>[2x]MGHHHHHHMVK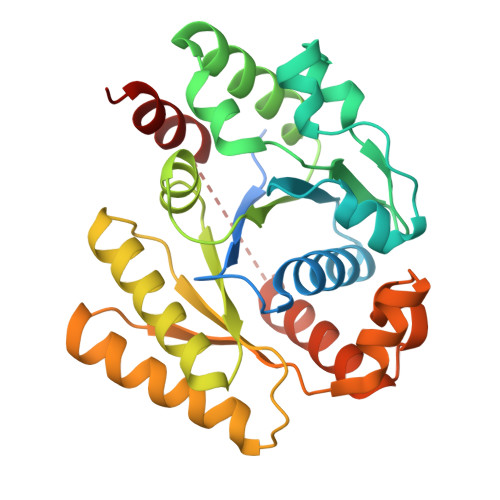DQAEQLRLKLSRLRQQPSPRTIAVTSGKGGVGKSNVSLNFSLSLSKLGFRVLLLDMDIGMGNIDILLGESSSLALADWFSARLPLSELVKSGPEHLSYIAGGTGAAQWQGLDTASIDRFLTELQAVASQYDYLIFDMGAGASGERLYFLKSVDDVFVVTTPEPTAMTDAYAMMKYMHAAGSEAPFSVIVNRAGKEREGYEVFERLKHVTGRFLNKDIALLGIIPEDRTVARAVVSQTPFVLLDPAAKASKAVRQMAFRYAPQREEGTERASRFFAKLRQLFLER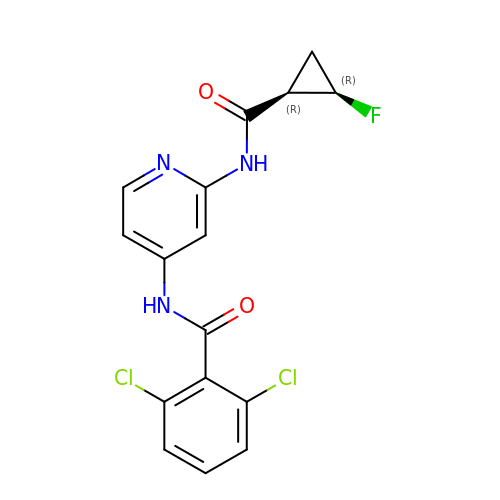2,6-dichloro-N-[2-({[(1R,2R)-2-fluorocyclopropyl]carbonyl}amino)pyridin-4-yl]benzamide | C16 H12 Cl2 F N3 O2 | RBNYBLHXBHWSCZ-JOYOIKCWSA-N>SNAMPKTLTEKLNAIKAAGKGIFVPYIMAGDHEKGLDGLAETIHFLEDLGVSAIEVGIPFSDPVADGPVIEEAGLRSLAHGTSTQALVETLKTIETEIPLVIMTYFNPLFQYGVENFVKDLADTAVKGLIIPDLPHEHANFVEPFLANTDIALIPLVSLTTGIERQKELIEGAEGFIYAVAINGVTGKSGNYRADLDKHLAQLHQVADIPVLTGFGVSSQADLERFNAVSDGVIVGSKIVKALHQGEPIQDFIRQAVAYQK[10x]

Tryptophan synthase is a key enzyme in l-tryptophan biosynthesis in plants, fungi and bacteria. The enzyme is composed of two catalytic units, TrpA (α subunit) and TrpB (β subunit), that associate into a functional heterotetrameric αββα hydrolyase complex (TrpAB). The enzyme catalyzes two reactions: the α subunit converts 1-C-(indol-3-yl)glycerol 3-phosphate (IGP) to indole and d-glyceraldehyde 3-phosphate, while the β subunit condenses indole with l-serine to give l-tryptophan, with pyridoxal 5′-phosphate (PLP) functioning as a cofactor. The Streptococcus pneumoniae subunit α (SpTrpA) studied in the present work is a 258-residue protein which in its monomeric form assumes the canonical (β/α)8 TIM-barrel fold with three additional helices (Michalska et al., 2019).

We have determined the crystal structure of S. pneumoniae TrpA, the α subunit of tryptophan synthase, a key enzyme in tryptophan biosynthesis, and have discovered that it exists in solution and in the crystal as a very unusual dimer formed by swapping the N-terminal H0–S1–H1–S2 portion of the TIM-barrel core. The dimeric fraction of the monomer–dimer mixture was crystallized in the monoclinic space group P21 with ten chains of SpTrpA in the asymmetric unit. The structure of SpTrpA was solved by single-wavelength anomalous X-ray diffraction (SAD) phasing and refined to 2.54 Å resolution. Moreover, many of the previous examples with accidental TIM-barrel involvement in oligomerization are not bona fide 3D domain-swapping cases because the monomeric form does not exist. In the domain-swapping of SpTrpA, the N-terminal structural elements (N)–H0–S1–H1–S2 (with the sequence Mse1–Asp59) are contributed by the complementary subunit. The linker or hinge region comprises the mostly hydrophobic Ile55–Gly64 decapeptide. The hinge-loop region involved in the domain swapping is the only part that adopts a different conformation in the monomeric and domain-swapped forms. Thus, the open interface seems to be stabilized mostly by hydrophobic interactions. The only visible change is in the conformation of the short linker (Ile55–Asp64) connecting the swapped domains. The active site in each TIM barrel is restored and two α chains now contribute residues to each active site in the dimer. Since there is no corresponding ligand in the active-site pocket in our structure, we cannot confirm the exact role of the disordered flexible loop L6 (residues ∼180–190) in ligand binding.> AGCGCCUGGACUUAAAGCCAUUGCACU;> GGCGGCUUUAAGUUGACGAGGGCAGGGUUAAACGAGACAUCGGCGAGUGCC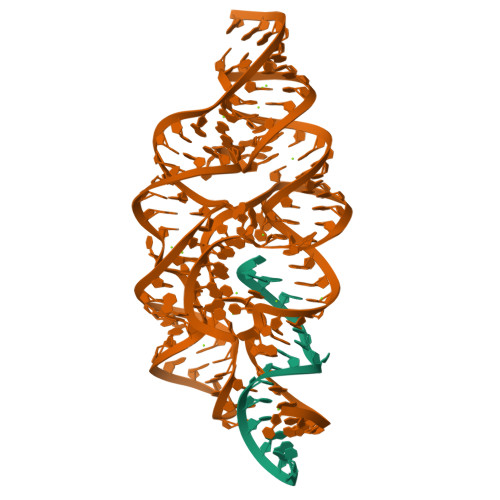CUGCGGUCUUCCUGCGACCGUUAGAGGACUGGUAAAACCACAGGCGACUGUGGCAUAGAGCAGUCCGGGCAGGAA> RSMGNEFEDYCLKRELLMGIFEMGWEKPSPIQEESIPIALSGRDILARAKNGTGKSGAYLIPLLERLDLKKDNIQAMVIVPTRELALQVSQICIQVSKHMGGAK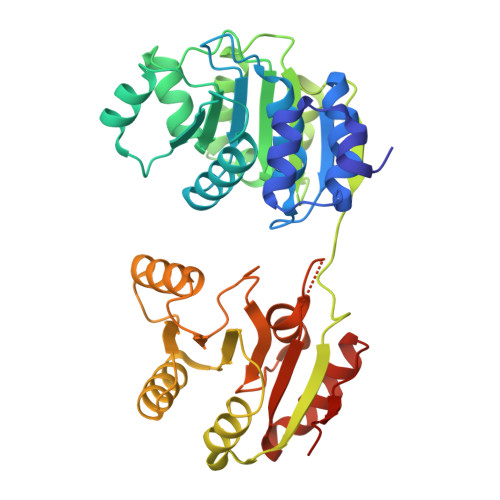VMATTGGTNLRDDIMRLDDTVHVVIATPGRILDLIKKGVAKVDHVQMIVLDEADKLLSQDFVQIMEDIILTLPKNRQILLYSATFPLSVQKFMNSHLQKPYEINLMEELTLKGVTQYYAYVTERQKVHCLNTLFSRLQINQSIIFCNSSQRVELLAKKISQLGYSCFYIHAKMRQEHRNRVFHDFRNGLCRNLVCTDLFTRGIDIQAVNVVINFDFPKLAETYLHRIGRSGRFGHLGLAINLITYDDRFNLKSIEEQLGTEIKPIPSNIDKSLY>[2x]MQLELSTCVFLCLLPLGFSAIRRYYLGAVELSWDYRQSELLRELHVDTRFPATAPGALPLGPSVLYKKTVFVEFTDQLFSVARPRPPWMGLLGPTIQAEVYDTVVVTLKNMASHPVSLHAVGVSFWKSSEGAEYEDHTSQREKEDDKVLPGKSQTYVWQVLKENGPTASDPPCLTYSYLSHVDLVKDLNSGLIGALLVCREGSLTRERTQNLHEFVLLFAVFDEGKSWHSARNDSWTRAMDPAPARAQPAMHTVNGYVNRSLPGLIGCHKKSVYWHVIGMGTSPEVHSIFLEGHTFLVRHHRQASLEISPLTFLTAQTFLMDLGQFLLFCHISSHHHGGMEAHVRVESCAEEPQLRRKADEEEDYDDNLYDSDMDVVRLDGDDVSPFIQIRSVAKKHPKTWVHYIAAEEEDWDYAPLVLAPDDRSYKSQYLNNGPQRIGRKYKKVRFMAYTDETFKTREAIQHESGILGPLLYGEVGDTLLIIFKNQASRPYNIYPHGITDVRPLYSRRLPKGVKHLKDFPILPGEIFKYKWTVTVEDGPTKSDPRCLTRYYSSFVNMERDLASGLIGPLLICYKESVDQRGNQIMSDKRNVILFSVFDENRSWYLTENIQRFLPNPAGVQLEDPEFQASNIMHSINGYVFDSLQLSVCLHEVAYWYILSIGAQTDFLSVFFSGYTFKHKMVYEDTLTLFPFSGETVFMSMENPGLWILGCHNSDFRNRGMTALLKVSSCDKNTGDYYEDSYEDISAYLLSKNNAIEPRSFAQNSRPPSASAPKPPVLRRHQRDISLPTFQPEEDKMDYDDIFSTETKGEDFDIYGEDENQD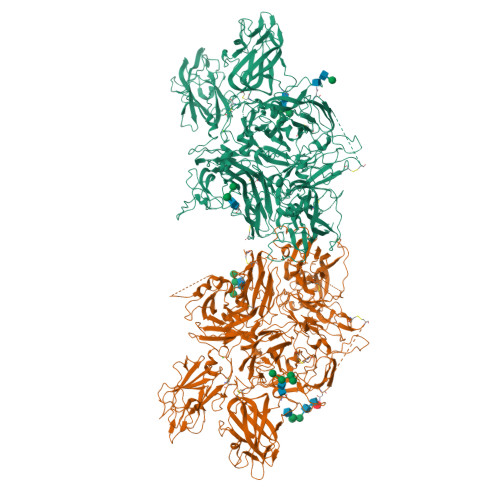PRSFQKRTRHYFIAAVEQLWDYGMSESPRALRNRAQNGEVPRFKKVVFREFADGSFTQPSYRGELNKHLGLLGPYIRAEVEDNIMVTFKNQASRPYSFYSSLISYPDDQEQGAEPRHNFVQPNETRTYFWKVQHHMAPTEDEFDCKAWAYFSDVDLEKDVHSGLIGPLLICRANTLNAAHGRQVTVQEFALFFTIFDETKSWYFTENVERNCRAPCHLQMEDPTLKENYRFHAINGYVMDTLPGLVMAQNQRIRWYLLSMGSNENIHSIHFSGHVFSVRKKEEYKMAVYNLYPGVFETVEMLPSKVGIWRIECLIGEHLQAGMSTTFLVYSKKCQTPLGMASGHIRDFQITASGQYGQWAPKLARLHYSGSINAWSTKEPFSWIKVDLLAPMIIHGIKTQGARQKFSSLYISQFIIMYSLDGKKWQTYRGNSTGTLMVFFGNVDSSGIKHNIFNPPIIARYIRLHPTHYSIRSTLRMELMGCDLNSCSMPLGMESKAISDAQITASSYFTNMFATWSPSKARLHLQGRSNAWRPQVNNPKEWLQVDFQKTMKVTGVTTQGVKSLLTSMYVKEFLISSSQDGHQWTLFFQNGKVKVFQGNQDSFTPVVNSLDPPLLTRYLRIHPQSWVHQIALRMEVLGCEAQDLY> MSFVAAAVSRSGPAVVRIDTETVVTRRTDPILDDPFFQEFFGRSFPVPPRERRIAGQGSGFIIDNSGIILTNAHVVDGASKVVVTLRDGRTFDGQVRGTDEVTDLAVVKIEPQGSALPVAPLGTSSNLQVGDWAIAVGNPVGLDNTVTLGIISTLGRSAAQAGIPDKRVEFIQTDAAINPG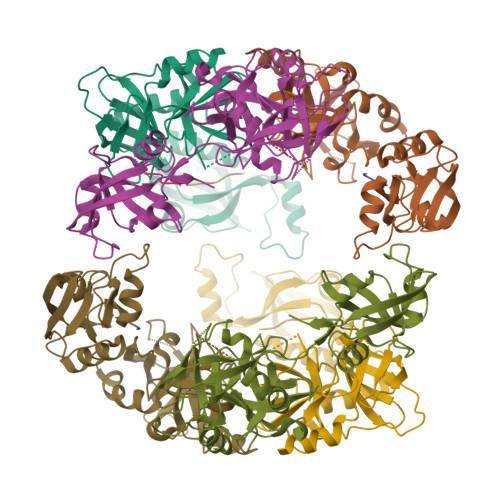NSGGPLLNARGEVIGINTAIRADATGIGFAIPIDQAKAIQNTLAAGGTVPHPYIGVQMMNITVDQAQQNNRNPNSPFIIPEVDGILVMRVLPGTPAERAGIRRGDVIVAVDGTPISDGARLQRIVEQAGLNKALKLDLLRGDRRLSLTVQTAQLRNPTSLEHHHHHH>[6x]GSESLLYGYFLDSWLDGTASEEMMR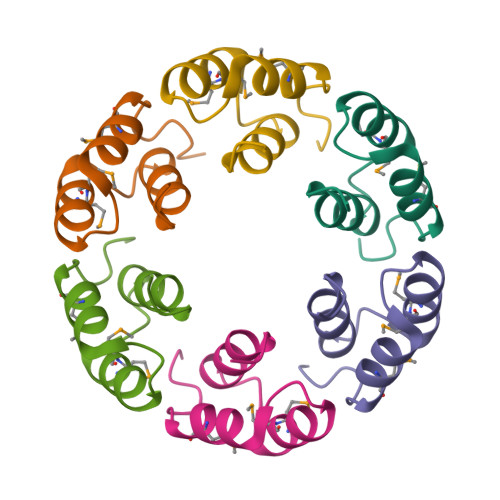VAVNAGDLTQEEADKIMSYPWGAWND3-({4-[(5-CHLORO-1,3-BENZODIOXOL-4-YL)AMINO]PYRIMIDIN-2-YL}AMINO)BENZAMIDE 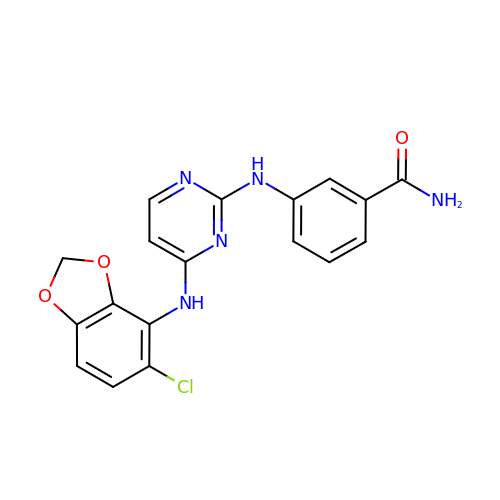| C18 H14 Cl N5 O3 | ZVQZIVCQLFGXFZ-UHFFFAOYSA-N> MDVRQVLHMKGGAGENSYAMNSFIQRQVISITKPITEAAITALYSGDTVTTRLAIADLGCSSGPNALFAVTELIKTVEELRKKMGRENSPEYQIFLNDLPGNDFNAIFRSLPIENDVDGVCFINGVPGSFYGRLFPRNTLHFIHSSYSLMWLSQVPIGIESNKGNIYMANTCPQSVLNAYYKQFQEDHALFLRCRAQEVVPGGRMVLTILGRRSEDRASTECCLIWQ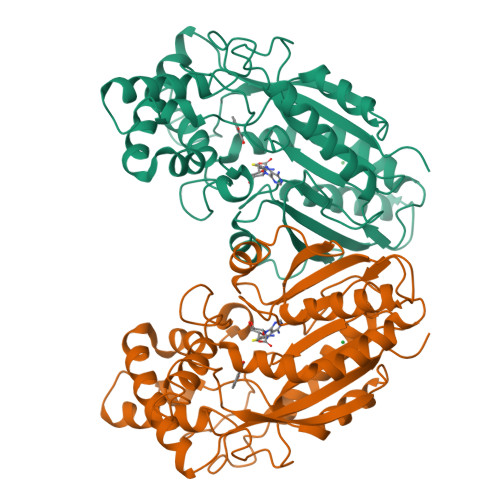LLAMALNQMVSEGLIEEEKMDKFNIPQYTPSPTEVEAEILKEGSFLIDHIEASEIYWSSCTKDGDGGGSVEEEGYNVARCMRAVAEPLLLDHFGEAIIEDVFHRYKLLIIERMSKEKTKFINVIVSLIRKSD>CNGRCGVRSSSRTPSDKPVAHVVANPQAEGQLQWLNRRANALLANGVELRDNQLVVPSEGLYLIYSQVLFKGQGCPSTHVLLTHTISRIAVSYQTKVNLLSAIKSPCQRETPEGAEAKPWYEPIYLGGV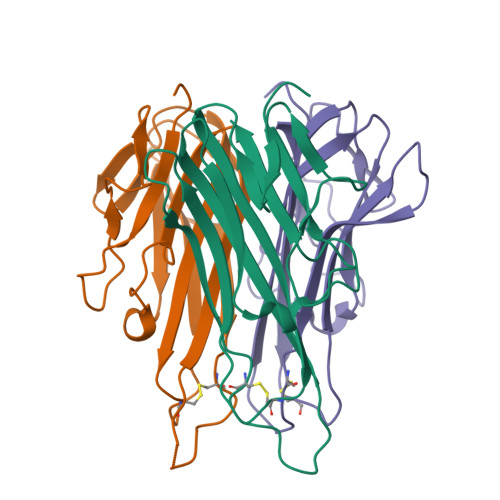FQLEKGDRLSAEINRPDYLDFAESGQVYFGIIAL[3x]> SHGNIDLGFIYTMGAHTVPELVQNFTKVESHKDITFSFFQGATKSIIPDLKNEKFDLAICSYVENEPDIEFLPLTKQELVVVVAENHPLAKYDSIDLQDTADYSYIFFSDTSGLRPLIDSLFAEINIQPKIGCYVEEDTAMVGLVSVDYGISI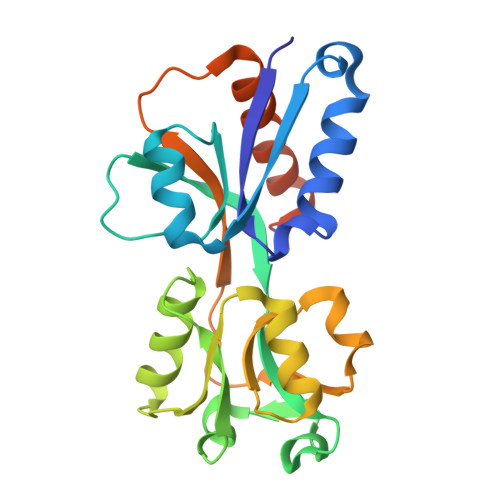MPKISSLAHYNVKVLSINEPKHDRFIYLASLKNHYISPASKAFKDFALRYGKKHFLRENLYFQGLEHHHHHHH N-(1-{[4-(aminomethyl)phenyl]sulfonyl}piperidin-4-yl)-5-cyclopropyl-1,2-oxazole-3-carboxamide 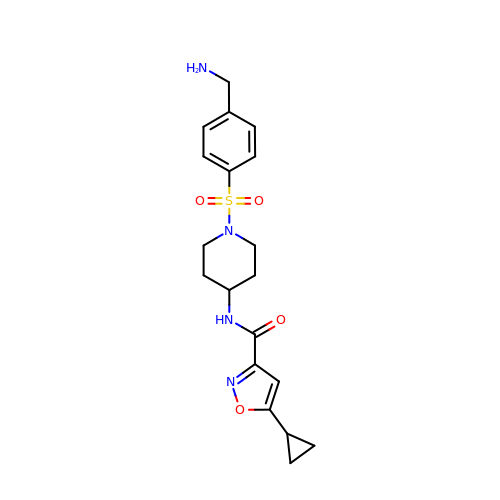| C19 H24 N4 O4 S | VYWACYQGNDEUMV-UHFFFAOYSA-N> MAGRARSGLLLLLLGLLALQSSCLAFRSPLSVFKRFKETTRSFSNECLGTIGPVTPLDASDFALDIRMPGVTPKESDTYFCMSMRLPVDEEAFVIDFKPRASMDTVHHMLLFGCNMPSSTGSYWFCDEGTCTDKANILYAWARNAPPTRLPKGVGFRVGGETGSKYFVLQVHYGDISAFRDNHKDCSGVSVHLTRVPQPLIAGMYLMMSVDTVIPPGEKVVNADISCQYKMYPMHVFA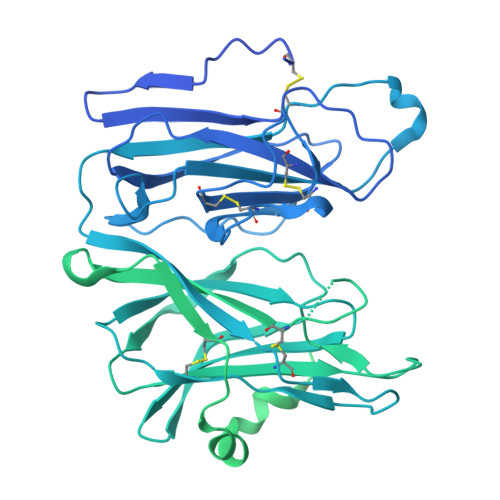YRVHTHHLGKVVSGYRVRNGQWTLIGRQNPQLPQAFYPVEHPVDVTFGDILAARCVFTGEGRTEATHIGGTSSDEMCNLYIMYYMEAKYALSFMTCTKNVAPDMFRTIPAEANIPIPVKPDMVMMHGHHKEAENKEKSALMQQPKQGEEEVLEQGDFYSLLSKLLGEREDVHVHKYNPTEKTESGSDLVAEIANVVQKKDLGRSDAREGAEHEEWGNAILVRDRIHRFHQLESTLRPAESRAFSFQQPGEGPWEPEPSGDFHVEEELDWPGVYLLPGQVSGVALDSKNNLVIFHRGDHVWDGNSFDSKFVYQQRGLGPIEEDTILVIDPNNAEILQSSGKNLFYLPHGLSIDTDGNYWVTDVALHQVFKLDPHSKEGPLLILGRSMQPGSDQNHFCQPTDVAVEPSTGAVFVSDGYCNSRIVQFSPSGKFVTQWGEESSGSSPRPGQFSVPHSLALVPHLDQLCVADRENGRIQCFKTDTKEFVREIKHASFGRNVFAISYIPGFLFAVNGKPYFGDQEPVQGFVMNFSSGEIIDVFKPVRKHFDMPHDIVASEDGTVYIGDAHTNTVWKFTLTEKMEHRSVKKAGIEVQEIKEAEAVVEPKVENKPTSSELQKMQEKQKLSTEPGSGVSVVLITTLLVIPVLVLLAIVMFIRWKKSRAFGDHDRKLESSSGRVLGRFRGKGSGGLNLGNFFASRKGYSRKGFDRVSTEGSDQEKDEDDGTESEEEYSAPLPKPAPSS Complex I (NADH:ubiquinone (UQ) oxidoreductase) is the first and the largest enzyme of the respiratory chain, catalysing the transfer of two electrons from NADH to UQ, coupled to the translocation of four protons across the bacterial or inner mitochondrial membrane. In bacterial complex I the 14 “core” subunits, necessary and sufficient for complex I function, are shared equally between the peripheral and membrane arms, together forming an L-shaped molecule. All known co-factors of complex I reside in the PA: the primary electron acceptor flavin-mononucleotide (FMN) is connected by the redox chain of seven Fe–S clusters to the quinone-binding site (Q-site) at the interface with the membrane domain. In this work we address this question by building and analyzing atomic structures of nine different conformational states of complex I, which were obtained by X-ray crystallography and single-particle cryo-EM.

Aureothin, pyridaben and piericidin A are the most potent inhibitors of T. thermophilus complex I, while rotenone is less effective than it is with mammalian enzyme. All Q-like ligands studied here display a similar pattern of interactions at the deepest end of the Q-cavity, with the headgroup about 12 Å away from cluster N2. A shared feature between all ligands bound in the Q-site is a hydrogen bond interaction of a ketone group from the quinone ring with the conserved and essential for complex I activity Y87416,36. Piericidin A shows similar interactions with the addition of a hydrogen bond between Q2268 and the distal carbonyl group of its tail. In these structures quinone-like compounds are bound in the main “deep” site within the cavity, where quinone can effectively accept electrons from cluster N2. Most dramatic changes are caused by DQ binding, whilst Q-like inhibitors alter complex I conformation consistently in a similar way but to a lesser degree, to states intermediate between CXIINT and CXIDQ. The overlap analysis (OA) (technique described below) shows that transitions from CXIINT structure to CXIAUT and CXIPYR involve relatively minor PA rotation component (mode 8), which is much stronger for CXIPIE structure and is accompanied in addition by a bending motion (mode 7) for CXIDQ structure. That is, Q-site binding by DQ, and to some extent Q-like inhibitors studied here, appears to shift the conformational energy minimum towards the CXIMN-like state, allowing us to observe such conformations in crystals.

>[2x]MTGPILSGLDPRFERTLYAHVGKEGSWTLDYYLRHGGYETAKRVLKEKTPDEVIEEVKRSGLRGRGGAGFPTGLKWSFMPKDDGKQHYLICNADESEPGSFKDRYILEDVPHLLIEGMILAGYAIRATVGYIYVRGEYRRAADRLEQAIKEARARGYLGKNLFGTDFSFDLHVHRGAGAYICGEETALMNSLEGLRANPRLKPPFPAQSGLWGKPTTINNVETLASVVPIMERGADWFAQMGTEQSKGMKLYQISGPVKRPGVYELPMGTTFRELIYEWAGGPLEPIQAIIPGGSSTPPLPFTEEVLDTPMSYEHLQAKGSMLGTGGVILIPERVSMVDAMWNLTRFYAHESCGKCTPCREGVAGFMVNLFAKIGTGQGEEKDVENLEALLPLIEGRSFCPLADAAVWPVKGSLRHFKDQYLALAREKRPVPRPSLWR;>[2x]MGFFDDKQDFLEETFAKYPPEGRRAAIMPLLRRVQQEEGWIRPERIEEIARLVGTTPTEVMGVASFYSYYQFVPTGKYHLQVCATLSCKLAGAEELWDYLTETLGIGPGEVTPDGLFSVQKVECLGSCHTAPVIQVNDEPYVECVTRARLEALLAGLRAGKRLEEIELPGKCGHHVHEVEV;>[2x]MVRVKVNDRIVEVPPGTSVMDAVFHAGYDVPLFCSEKHLSPIGACRMCLVRIGLPKKGPDGKPLLNEKGEPEIQWQPKLAASCVTAVADGMVVDTLSDVVREAQAGMVEFTLLNHPLDCPTCDKGGACELQDRTVEYGLYEKYYQKGPLELPVYTRFEFTRRHVDKHHPLSPFVILDRERCIHCKRCVRYFEEVPGDEVLDFIERGVHTFIGTMDFGLPSGFSGNITDICPVGALLDLTARFRARNWEMEETPTTCALCPVGCGITADTRSGELLRIRAREVPEVNEIWICDAGRFGHEWADQNRLKTPLVRKEGRLVEATWEEAFLALKEGLKEARGEEVGLYLAHDATLEEGLLASELAKALKTPHLDFQGRTAAPASLFPPASLEDLLQADFALVLGDPTEEAPILHLRLSEFVRDLKPPHRYNHGTPFADLQIKERMPRRTDKMALFAPYRAPLMKWAAIHEVHRPGEEREILLALLGDKEGSEMVAKAKEAWEKAKNPVLILGAGVLQDTVAAERARLLAERKGAKVLAMTPAANARGLEAMGVLPGAKGASWDEPGALYAYYGFVPPEEALKGKRFVVMHLSHLHPLAERYAHVVLPAPTFYEKRGHLVNLEGRVLPLSPAPIENGEAEGALQVLALLAEALGVRPPFRLHLEAQKALKARKVPEAMGRLSFRLKELRPKERKGAFYLRPTMWKAHQAVGKAQEAARAELWAHPETARAEALPEGAQVAVETPFGRVEARVVHREDVPKGHLYLSALGPAAGLRVEGRVLVPAGGEA;>MREEFLEEIPLDAPPEEAKELRTEVMTLNVGPQHPSTHGVLRLMVTLSGEEVLEVVPHIGYLHTGFEKTMEHRTYLQNITYTPRMDYLHSFAHDLAYALAVEKLLGAVVPPRAETIRVILNELSRLASHLVFLGTGLLDLGALTPFFYAFRERETILDLFEWVTGQRFHHNYIRIGGVKEDLPEEFVPELKKLLEVLPHRIDEYEALFAESPIFYERARGVGVIPPEVAIDLGLTGGSLRASGVNYDVRKAYPYSGYETYTFDVPLGERGDVFDRMLVRIREMRESVKIIKQALERLEPGPVRDPNPQITPPPRHLLETSMEAVIYHFKHYTEGFHPPKGEVYVPTESARGELGYYIVSDGGSMPYRVKVRAPSFVNLQSLPYACKGEQVPDMVAIIASLDPVMGDVDR[2x];>[2x]MRLERVLEEARAKGYPIEDNGLGNLWVVLPRERFKEEMAHYKAMGFNFLADIVGLDYLTYPDPRPERFAVVYELVSLPGWKDGDGSRFFVRVYVPEEDPRLPTVTDLWGSANFLEREVYDLFGIVFEGHPDLRKILTPEDLEGHPLRKDYPLGETPTLFREGRYIIPAEFRAALTGKDPGLTFYKGGSRKGYRSLWADLKKAREVKG;>MALKDLFERDVQELEREGILFTTLEKLVAWGRSNSLWPATFGLACCAIEMMASTDARNDLARFGSEVFRASPRQADVMIVAGRLSKKMAPVMRRVWEQMPDPKWVISMGACASSGGMFNNYAIVQNVDSVVPVDVYVPGCPPRPEALIYAVMQLQKKVRGQAYNERGERLPPVAAWKRTRG[2x];>MSASSERELYEAWVELLSWMREYAQAKGVRFEKEADFPDFIYRMERPYDLPTTIMTASLSDGLGEPFLLADVSPRHAKLKRIGLRLPRAHIHLHAHYEPGKGLVTGKIPLTKERFFALADRAREALAFA[2x];>MTLKALAQSLGITLKYLFSKPVTVPYPDAPVALKPRFHGRHVLTRHPNGLEKCIGCSLCAAACPAYAIYVEPAENDPENPVSAGERYAKVYEINMLRCIFCGLCEEACPTGAIVLGYDFEMADYEYSDLVYGKEDMLVDVVGTKPQRREAKRTGKPVKVGYVVPYVRPELEGFKAPTEGGKR[2x];>MAPIQEYVGTLIYVGVALFIGVAALLVGALLGPKKPGRAKLMPYESGNDPAGEVKRFPVHFYVVAMLFILFDVEVAFLWPYAVSAGGLGLYGFLGVLAFTLLLFVGFLYEWWKGVMRWH[2x];>MTWSYPVDPYWMVALKALLVVVGLLTAFAFMTLIERRLLARFQVRMGPNRVGPFGLLQPLADAIKSIFKEDIVVAQADRFLFVLAPLISVVFALLAFGLIPFGPPGSFFGYQPWVINLDLGILYLFAVSELAVYGIFLSGWASGSKYSLLGSLRSSASLISYELGLGLALLAPVLLVGSLNLNDIVNWQKEHGWLFLYAFPAFLVYLIASMAEAARTPFDLPEAEQELVGGYHTEYSSIKWALFQMAEYIHFITASALIPTLFLGGWTMPVLEVPYLWMFLKIAFFLFFFIWIRATWFRLRYDQLLRFGWGFLFPLALLWFLVTALVVALDLPRTYLLYLSALSFLVLLGAVLYTPKPARKGGGA[2x];>[2x]MSLLEGLALFLLLLSGVLVVTLRNAIHAALALILNFLVLAGVYVALDARFLGFIQVIVYAGAIVVLFLFVIMLLFAAQGEIGFDPLVRSRPLAALLALGVAGILAAGLWGLDLAFTQDLKGGLPQALGPLLYGDWLFVLLAVGFLLMAATVVAVALVEPGKASRAKEAEKREEVAR;>MSYLLTSALLFALGVYGVLTRRTAILVFLSIELMLNAANLSLVGFARAYGLDGQVAALMVIAVAAAEVAVGLGLIVAIFRHRESTAVDDLSELRG[2x];>MALLGTILLPLLGFALLGLFGKRMREPLPGVLASGLVLASFLLGAGLLLSGGARFQAEWLPGIPFSLLLDNLSGFMLLIVTGVGFLIHVYAIGYMGGDPGYSRFFAYFNLFIAMMLTLVLADSYPVMFIGWEGVGLASFLLIGFWYKNPQYADSARKAFIVNRIGDLGFMLGMAILWALYGTLSISELKEAMEGPLKNPDLLALAGLLLFLGAVGKSAQIPLMVWLPDAMAGPTPVSALIHAATMVTAGVYLIARSSFLYSVLPDVSYAIAVVGLLTAAYGALSAFGQTDIKKIVAYSTISQLGYMFLAAGVGAYWVALFHVFTHAFFKALLFLASGSVIHALGGEQDVRKMGGLWKHLPQTRWHALIGALALGGLPLLSGFWSKDAILAATLTYPFGGVGFYVGALLVAVLTAMYAMRWFVLVFLGEERGHHHPHEAPPVMLWPNHLLALGSVLAGYLALPHPLPNVLEPFLKPALAEVEAHHLSLGAEWGLIALSAAVALLGLWAGFVFFQRKVFPAWYLAFEAASREAFYVDRAYNALIVNPLKALAEALFYGDRGLLSGYFGLGGAARSLGQGLARLQTGYLRVYALLFVLGALLLLGVMRW[2x];>MVVLAVLLPVVFGALLLLGLPRALGVLGAGLSFLLNLYLFLTHPGGVAHAFQAPLLPGAGVYWAFGLDGLSALFFLTIALTVFLGALVARVEGRFLGLALLMEGLLLGLFAARDLLVFYVFFEAALIPALLMLYLYGGEGRTRALYTFVLFTLVGSLPMLAAVLGARLLSGSPTFLLEDLLAHPLQEEAAFWVFLGFALAFAIKTPLFPLHAWLPPFHQENHPSGLADALGTLYKVGVFAFFRFAIPLAPEGFAQAQGLLLFLAALSALYGAWVAFAAKDFKTLLAYAGLSHMGVAALGVFSGTPEGAMGGLYLLAASGVYTGGLFLLAGRLYERTGTLEIGRYRGLAQSAPGLAALALILFLAMVGLPGLSGFPGEFLTLLGAYKASPWLAALAFLSVIASAAYALTAFQKTFWEEGGSGVKDLAGAEWGFALLSVLALLLMGVFPGYFARGLHPLAEAFAKLLGGGA[2x];>[2x]MTLAILAVFSVALTLLGFVLPPQGVKRATLLGLALALASLLLTWGKPFAFGPYAVDGVSQVFTLLALLGALWTVGLVRSGRFEFYLLVLYAALGMHLLASTRHLLLMLVALEALSLPLYALATWRRGQGLEAALKYFLLGALAAAFFLYGAALFYGATGSLVLGAPGEGPLYALALGLLLVGLGFKAALAPFHFWTPDVYQGSPTPVVLFMATSVKAAAFAALLRVAAPPEALALLVALSVVVGNLAALAQKEAKRLLAYSSIAHAGYMALALYTGNAQALGFYLLTYVLATGLAFAVLSQISPDRVPLEALRGLYRKDPLLGLAFLVAMLSLLGLPPLAGFWGKYLAFAEAARAGAWGVLVLALVTSAVSAYYYLGLGLAVFARPEETPFRPGPPWARAAVVAAGVLLLALGLLPGLVLPALAAGG;>MVRVGMRAAPRVSLEALKAALGGLKLSEAKVYLITDWQDKRDQARYALLLHTGKKDLLVPDAFGPAFPGGEEALSELVGLLLAQGARRFYEAVVSPGEMTALLDLPPEELLKRVMAIANPTDPGIYLKRAA[2x]>[3x]MFNNEPLEQIDKELHDILADEEKRQRETINLIASENLTNGAVRECLGNRVSNKYSEGYPKKRYYGGNDFIDKIEELCQKRALEAFNVSDEEWGVNVQPLSGSAANVQALYALVGVKGKIMGMHLCSGGHLTHGFFDEKKKVS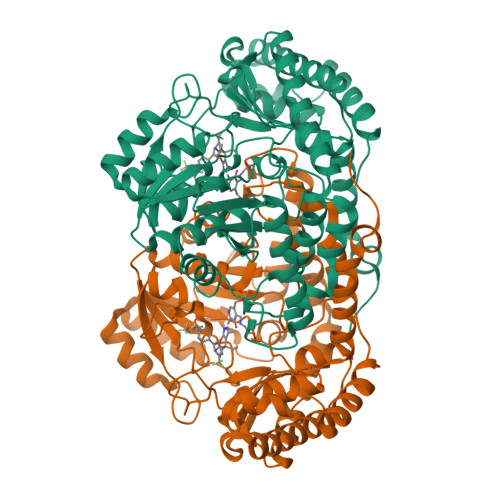ITSDMFESKLYKCNSQGYVDLDAVREMALSFKPKVIICGYTSYPRDIDYQQFRQICDEVNAYLFADISHISSFVACNILNNPFLHADVVTTTTHKILRGPRSALIFFNKKRNPGIEQKINSAVFPSFQGGPHNNKIAAVACQLKEVHSPAFKEYTQQVLLNSKALAKALISKQIDLVTNGTDNHLIVVDLRKFSITGSKLQETCNAINVSLNKNTIPSDVDAVSPSGVRIGTPAMTTRGAKEKDMEFIADVLARAIKITVDLQEQYGKKLVDFKKGLPGNAQLQQLKQEVVTWAGALPFP> MQEKSITIATEGGYAPWNFSGPGGKLDGFEIDLANALCEKMKAKCQIVAQNWDGIMPSLTGKKYDAIMAAMSVTPKRQEVIGFSIPYAAGINGFAVMGDSKLAEMPGLGETYSLDSQADAAKKAIADISSFLNGTTVGVQGSTTASTFLDKYFKGSVDIKEYKSVEEHNLDLTSGRLDAVLANATVLAAAIEKPEMKGAKLVGPLFSGGEFGVVAVGL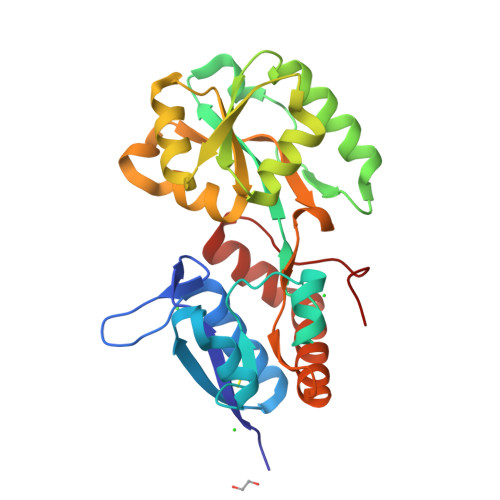RKEDTALKADFDAAIKAASEDGTIKTLSLKWFKVDVTPQHHHHHH(2E,6E)-2-fluoro-3,7,11-trimethyldodeca-2,6,10-trien-1-yl trihydrogen 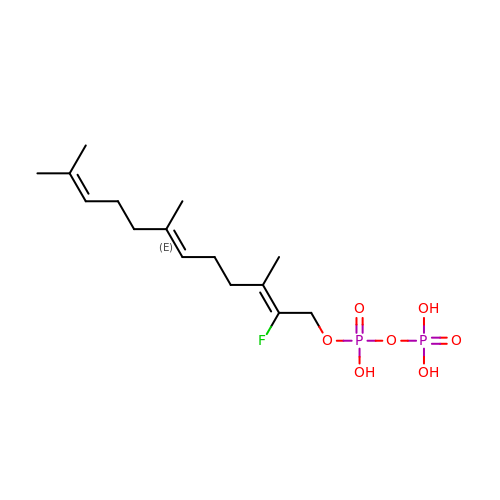diphosphate | C15 H27 F O7 P2 | DXHJZCKJWKWTCH-BBXOWAOSSA-N The light-producing reaction catalysed by the Renilla-type luciferase is one of the most widely used biochemical reactions in molecular and cell biology research. Here we track the role of dynamics in evolution, starting from the evolvable and thermostable ancestral protein AncHLD-RLuc which catalyses both dehalogenase and luciferase reactions. The regions encompassing the L9-α4 fragment and L14 loop are important structural elements that line the main access tunnels connecting the buried active site to the surrounding solvent. We conclude that the LUC activity benefits from conformational dynamics of the protein’s rigid scaffold to allow binding of a bulky substrate.

The most potent insertion variant, AncINS, has both an insertion and a substitution in the α4 helix. These mutations markedly improved substrate binding, linked to changes in dynamics of the cap domain, but not the putative catalytic pentad. The asymmetric unit of the crystal lattice of AncINS contains two monomers (chains A and B). Chain A has a structure similar to the AncHLD-RLuc template but features a π-helix bulge in the α4 helix where the L162 insertion and F163P substitution occurred. In AncINS chain B, the α4 helix is markedly distorted towards the α5 helix. In AncINS, the inserted L162 occupies the same position as the bulky F162 in AncHLD-RLuc, making the active site cavity of AncINS bigger than that of AncHLD-RLuc. The F163P substitution in AncINS disrupts the α4 helix because proline acts as a helix breaker, introducing a kink into the polypeptide backbone. The resulting distortion closes the main access tunnel in the chain B of AncINS. By contrast, we detected conformational flexibility of AncINS, accompanied by 1000-fold faster binding, based on determined k+1 and k-1. The HDX-MS profiles show that AncINS was deuterated more rapidly overall than the template AncHLD-RLuc, and that the modification of its α4 helix backbone leads to greater solvation and more pronounced dynamics, particularly in the cap domain region.

>[2x]TATGDEWWAKCKQVDVLDSEMSYYDSDPGKHKNTVIFLHGNPTSSYLWRNVIPHVEPLARCLAPDLIGMGKSGKLPNHSYRFVDHYRYLSAWFDSVNLPEKVTIVCHDWGSGLGFHWCNEHRDRVKGIVHMESVVSPLKGWESFPETARDILPQALRSEAGEEMVLKKNFFIERLLPSSIMRKLSEEEMDAYREPFVEPGESRRPTLTWPREIPIKGDGPEDVIEIVKSYNKWLSTSKDIPKLFINADPGFFSNAIKKVTKNWPNQKTVTVKGLHFLQEDSPEEIGEAIADFLNELTK> GSHMKNSVSVDLPGSMKVLVSKSSNADGKYDLIATVDALELSGTSDKNNGSGVLEGVKADASKVKLTISDDLGQTTLEVFKSDGSTLVSKKVTSKDKVLADV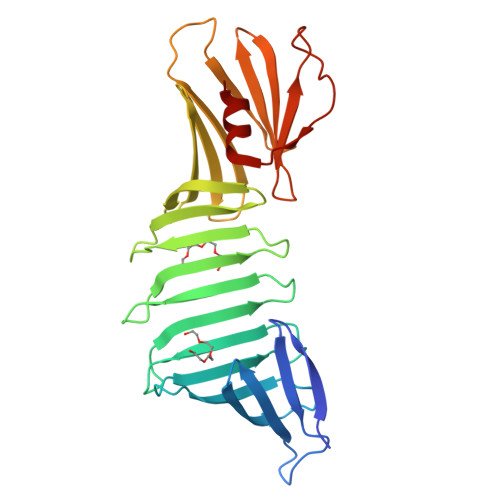KFNEKGEVSEKIITRADGTRLEYTGIKSDGSGKAKEVLKGYVLEGTLTAEKTTLVVKEGTVTLSKNISKSGAVSVELNDTDSSAATKKTAAWNSGTSTLTITVNSKKTKDLVFTSSNTITVQQYDSNGTSLEGSAVEITKLDEIKNALK> HSDPARRGQLSVCDSISEWVTAADKKTAVDMSGGTVTVLEKVPVSKGQLKQYFY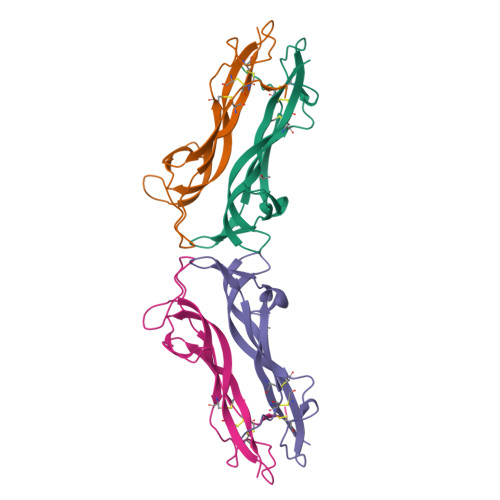ETKCNPMGYTKEGCRGIDKRHWNSQCRTTQSYVRALTMDSKKRIGWRFIRIDTSCVCTLTIKRGR;> YAEHKSHRGEVSVCDSESLWVTDKSSAIDIRGHQVTVLGEIKTQNSPVKQYFYETRCKEARPVKNGCRGIDDKHWNSQCKTSQTYVRALTSENNKLVGWRWIRIDTSCVCALSRKIGRT>SNASLKANFYKNRVCLNVLAGSVDNAADIYDAAEGHVLVGVLSKNYPDVDTAVEDMKKYSEVTNNAVSVGLGAGDPNQSMMVSLISQHVQPQHINQVFTGVATSRALAGQDKSIVNGLISPTGTVGMVKISTGPLSSRSEDAIVPVETAIAMLKDMGGSSVKYFPMGGL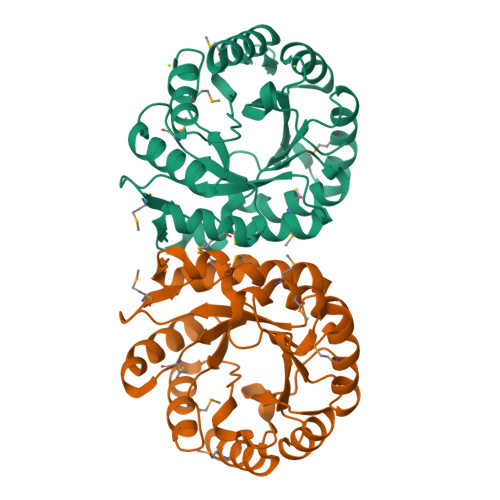ETREEFACVAKACADKDFWLEPTGGIDLENYEEIMQIALDAGVSKIIPHIYSSIIDKATGNTRPEDVKTLLDMTKKLLL[4x]> SGSGSGSGSGSEFNATQINEELYRLLEDTEILNQEITEGLLKGFEVPDAGVAIQLSKRDVVYPARILIIVLSEMWRFGLTKQSESFLAQVLTTIQKVVTQLKGNDLIPSGVFWLANVRELYSFVVFALNSILTEETFKNGMTDEEYKEYVSLVTELKDDFEALSYNIYNI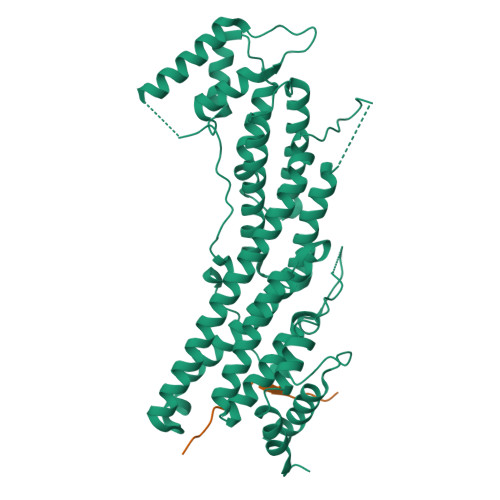WLKKLQKQLQKKAINAVVISESLPGFSAGETSGANTEEYTMDDILTFFNSIYWCMKSFHIENEVFHAVVTTLLNYVDAICFNELIMKRNFLSWKRGLQLNYNVTRLEEWCKTHGLTDGTECLQHLIQTAKLLQVRKYTIEDIDILRGICYSLTPAQLQKLISQYQVADYESPIPQEILRYVADIVKKEAALSSSGNDSKGHEHSSSIFITPETGPFTDPFSLIKTRKFDQVEAYIPAWLSLPSTKRIVDLVAQQVVQDGH;> GPGSSSSSIATTGSQESFVARPFKKGLNLHSIKVTSSTPKGSENLYFQ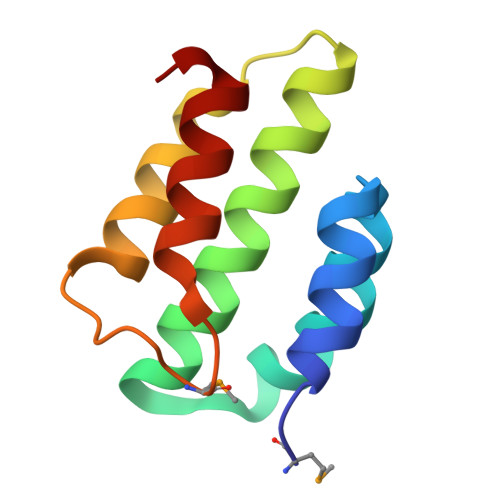>[2x]MVPDWEEVLGLWRAGRYYEVHEVLEPYWLKATGEERRLLQGVILLAAALHQRRLGRPGLRNLRKAEARLEGLPCPLMGLDWRSLLQEARRRLGA>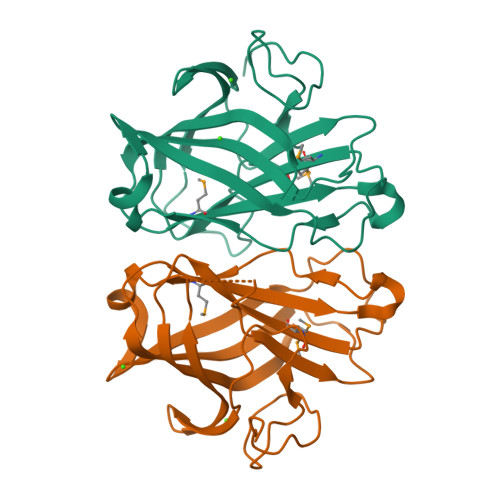GTEVEIPVVHDPKGEAVLPSVFEDGTRQGWDWAGESGVKTALTIEEANGSNALSWEFGYPEVKPSDNWATAPRLDFWKSDLVRGENDYVTFDFYLDPVRATEGAMNINLVFQPPTNGYWVQAPKTYTINFDELEEANQVNGLYHYEVKINVRDITNIQDDTLLRNMMIIFADVESDFAGRVFVDNVRFEGA[2x]> MSGSHHHHHHSSGIEGRGRLIKHRPAVQDERAVRIAVFVPGFRHDSPVYAMLCDGVERAVTQERATGRSIGLDIIEAGPNQALWREKLAHLAAEQRYRLIVSSNPALPHVLEPILRQFPLQRFLVLDAYAPQEHSLITFRYNQWEQAYLAGHLSALVSASAMRFANADKKIGLIA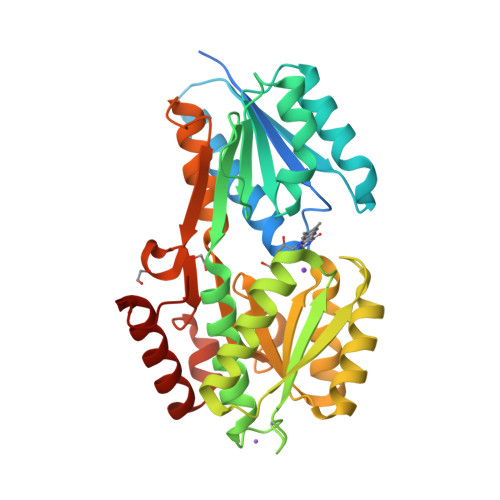GQSYPVMTQTIIPAFLAGARAVDPAFEVDVRVVGNWYDAAKSADLARILFHEGVDVMMPICGGANQGVLAAARELGFYVSWFDDNGYARAPGYVVGSSVMEQERLAYEQTLRCIRGELPSAGAWTLGVKDGYVRFIEEDPLYLQTVPEPIRVRQSALLRRIQSGELTLPVR> 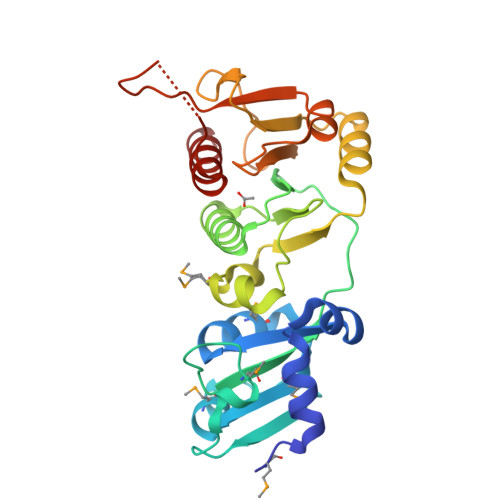SNAMLSANQIKFLRSLRERKYRLREQAFAVEGPKLVGEMLPFYRCRMLVGTAAMLRAVSTPHDAEVVELPESFDFKRISTQTTPQPLMAVFDLPAEPEPVVEGLTLLLDGVQDPGNVGTILRTADWFGIRHVWLGTGSADVFSPKVVQASMGALARVQPTPLKNTVDTLAYFRRQGIPVYGAFLDGQSLYEAPLPNFTEPAILVLGSEGRGISPEVAAEITDRLTIPASGLSVKGHTESLNVAIATAILCSEWRRRS> MGTPALDRAKLLKQYRKARKRLFMFDYDGTLTPIVKDPQAAIPSDRVLRTLKTLAADPRNAVWIISGRDQAFLDEWMGHIPELGLSAEHGCFIRQPRSDDWENLAESSDMGWQKEVMEVFQHFTERTQGSFIERKRVALTWHYRRADPEYGAFQARECRKMLEETVAKRWEVEVMAGKANLEVRPTFVNKGFIAARLVQEYGTDPAQAPEFVLCLGDDFTDEDMFRALKKSGLPAGHVFSVTVGASSKQTEASWHLLEPADVIGTISM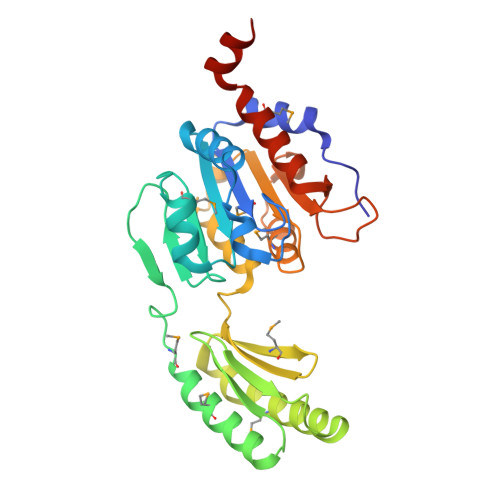LNNSSSAQEYLEHHHHHH> MGHHHHHHGSIESLCMNCYRNGTTRLLLTKIPFFREIIVSSFSCEHCGWNNTEIQSAGRIQDQGVRYTLTVRSQEDMNREVVKTDSATTRIPELDFEIPAFSQKGALTTVEGLISRAISGLEQDQPTRRAVEGAIAERIDEFIGKLKDLKQMASPFTLVIDDPSGNSFVENPHAPQKDNALVITYYDRTPQQAEMLGLQA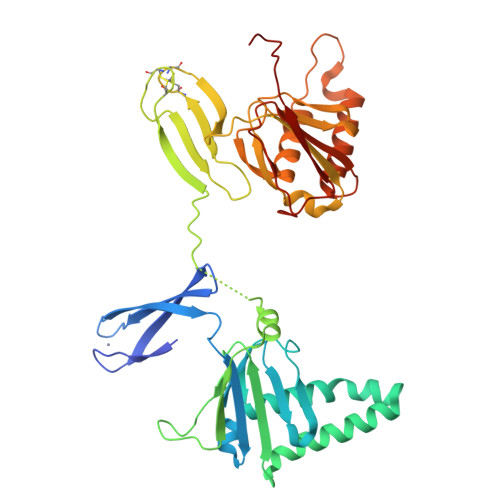EAPEEKAEEEDLRNEVLQFNTNCPECNAPAQTNMKLVQIPHFKEVIIMATNCENCGHRTNEVKSGGAVEPLGTRITLHITDPSDMTRDLLKSETCSVEIPELEFELGMAVLGGKFTTLEGLLKDIRELVTKNPFTLGDSSNPDQSEKLQEFSQKLGQIIEGKMKAHFIMNDPAGNSYLQNVYAPEDDPEMKVERYKRTFDQNEE>MEKRGVIDTWIDKHRSIYTAATRHAFVVSIRDGSVDLSSFRTWLGQDYLFVRRFVPFVASVLIRACKDSGESSDMEVVLGGIASLNDEIEWFKREGSKWDVDFSTVVPQRANQEYGRFLEDLMSSEVKYPVIMTAFWAIEAVYQESFAHCLEDGNKTPVELTGACHRWGNDGFKQYCSS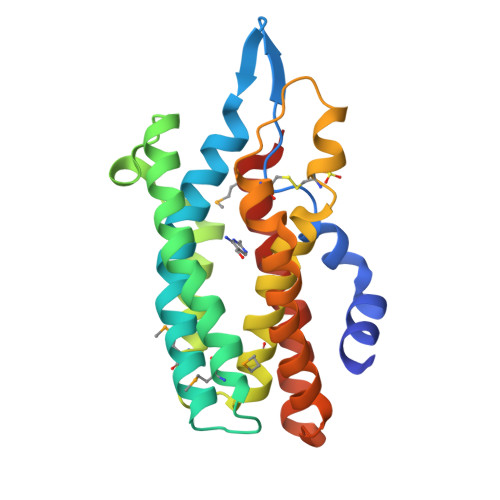VKNIAERCLENASGEVLGEAEDVLVRVLELEVAFWEMSRGGQ[2x]>MASPMFLPCVLVPNTRDCRPLTYQAAIPELRTPEELNPIIVTPPIQAIDQDRNIQPPSDRPGILYSILVGTPEDYPRFFHMHPRTAELSLLEPVNRDFHQKFDLVIKAEQDNGHPLPAFAGLHIEILDENNQSPYFTMPS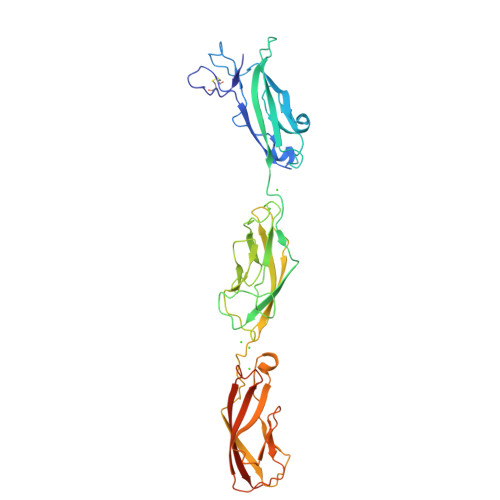YQGYILESAPVGATISDSLNLTSPLRIVALDKDIEDTKDPELHLFLNDYTSVFTVTQTGITRYLTLLQPVDREEQQTYTFSITAFDGVQESEPVIVNIQVMDANDNTPTFPEISYDVYVYTDMRPGDSVIQLTAVDADEGSNGEITYEILVGAQGDFIINKTTGLITIAPGVEMIVGRTYALTVQAADNAPPAERRNSICTVYIEVLPPNNQSPPRFLEHHHHHH[2x]> SNAMSQKLYNMKFAAVYLALIAKVERKGGKAESVHQVTSWLTGYEVSDV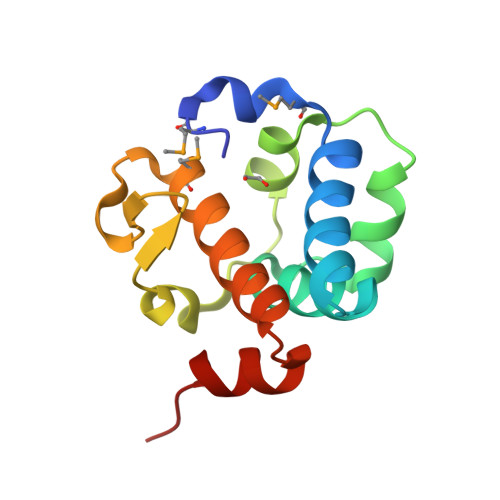LACLDRDVTYGDFFRQAPYYVPERIAITGKICGVRIEEIDDPLMQEIRRLDKLVDWLAKGKTSQQVLEKYEKHK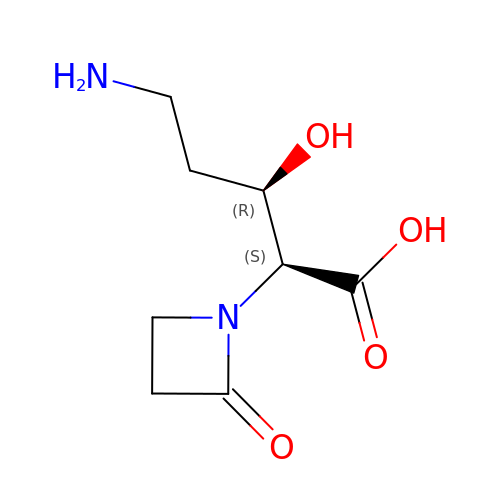5-AMINO-3-HYDROXY-2-(2-OXO-AZETIDIN-1-YL)-PENTANOIC ACID | C8 H14 N2 O4 | NMCINKPVAOXDJH-VDTYLAMSSA-N>[2x]SAGDHEPEFIGSPVAADEARSNWPKRYGRSTAAKKPDEEEELKARCHYRSAKVDNVVYCLGDDVYVKAGENEADYIGRITEFFEGTDQCHYFTCRWFFRAEDTVINSLVSISVDGHKHDPRRVFLSEEKNDNVLDCIISKVKIVHVDPNMDPKAK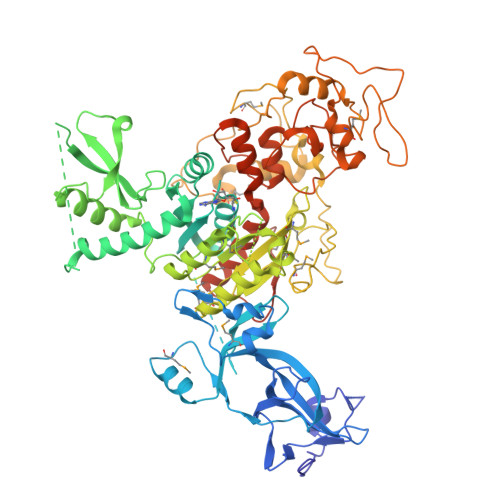AQLIESCDLYYDMSYSVAYSTFANISSENGQSGSDTASGISSDDVDLETSSSMPTRTATLLDLYSGCGGMSTGLCLGAALSGLKLETRWAVDFNSFACQSLKYNHPQTEVRNEKADEFLALLKEWAVLCKKYVQDVDSNLASSEDQADEDSPLDKDEFVVEKLVGICYGGSDRENGIYFKVQWEGYGPEEDTWEPIDNLSDCPQKIREFVQEGHKRKILPLPGDVDVICGGPPCQGISGFNRYRNRDEPLKDEKNKQMVTFMDIVAYLKPKYVLMENVVDILKFADGYLGKYALSCLVAMKYQARLGMMVAGCYGLPQFRMRVFLWGALSSMVLPKYPLPTYDVVVRGGAPNAFSQCMVAYDETQKPSLKKALLLGDAISDLPKVQNHQPNDVMEYGGSPKTEFQRYIRLSRKDMLDWSFGEGAGPDEGKLLDHQPLRLNNDDYERVQQIPVKKGANFRDLKGVRVGANNIVEWDPEIERVKLSSGKPLVPDYAMSFIKGKSLKPFGRLWWDETVPTVVTRAEPHNQVIIHPTQARVLTIRENARLQGFPDYYRLFGPIKEKYIQVGNAVAVPVARALGYCLGQAYLGESEGSDPLYQLPPSFTSVGGRTAGQARASPVGTPAGEVVEQ> MAKNTSCGVQLRIRGKVQGVGFRPFVWQLAQQLN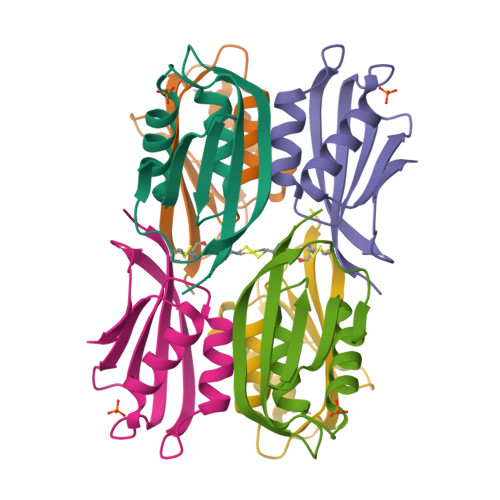LHGDVCNDGDGVEVRLREDPEVFLVQLYQHCPPLARIDSVEREPFIWSALPTEFTIR(1S)-1-(4-nitrophenyl)ethan-1-ol | C8 H9 N O3 | 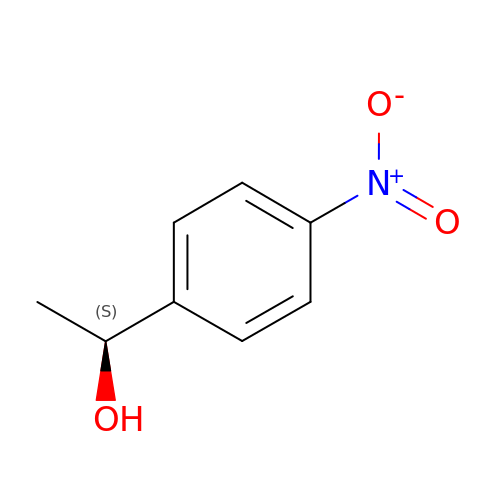CRJFHXYELTYDSG-LURJTMIESA-N> ASYLSVGYFNGGGDVTAGPGGDINKLDVTQITHLNYSFGLIYNDEKQETNPALKDPSRLHQIYLSPKVMADLQLLPVLRKQNPELKVLLSVGGWGARGFSGAAATAESRAVFIRSVQQVIKQYHLDGIDLDWEYPVNGAWGLVESQPADRANFTLLLAELHKALDKGKLLTIAVGANVKSPQEWVDVKGIAPYLDYINLMTYDMAYGTQYFNSNLYDSKQWPTVAAA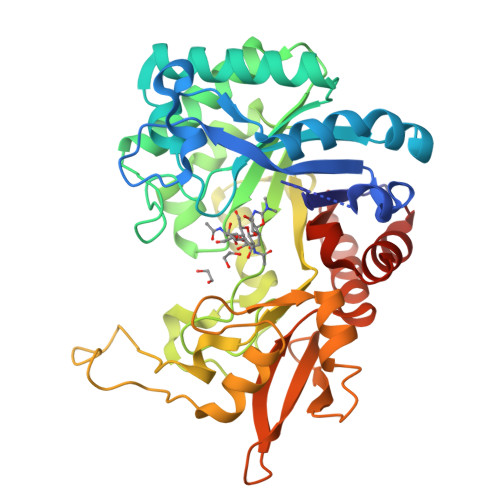DRYSANFVVDNYLAAGLKPAQLNLGIGFYGRVPKRATEPGIDWDKADAAKNPVTQPYFTARETAVFKAMGLDLTKDSYFKYNDIVSKLLNDPQRRFTAHWDSDAQVPYLTMKSAEGKPLFAISYENPRSVALKADYIKSKGLGGAMFWEYGADDNNRLAHQLAESLGINGGKQ> HHHHHHSSGLVPRGSHMTAQTVTGAVAAAQLGATLPHEHVIFGYPGYAGDVTLGPFDHAAALASCTETARALLARGIQTVVDATPNGCGRNPAFLREVSEATGLQILCATGFYYEGGGATTYFKFRASLGDAESEIYEMMRTEVTEGIAGTGIRAGVIKLASSRDAITPYEQLFFRAAARVQRETGVPIITHTQEGQQGPQQAELLTSLGADPARIMIGHMDGNTDPAYHRETLRHGVSIAFDRIGLQGMVGTPTDAERLSVLTTLLGEGYADRLLLSHDSIWHWLGRPPAIPEAALPA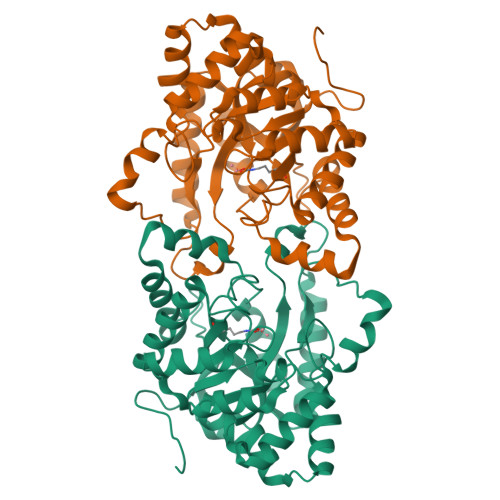VKDWHPLHISDDILPDLRRRGITEEQVGQMTVGNPARLFG> GAGCAGACCAG;> ACTCCACTCA;> CTAGT;> TCTGAGTGGGGTCTG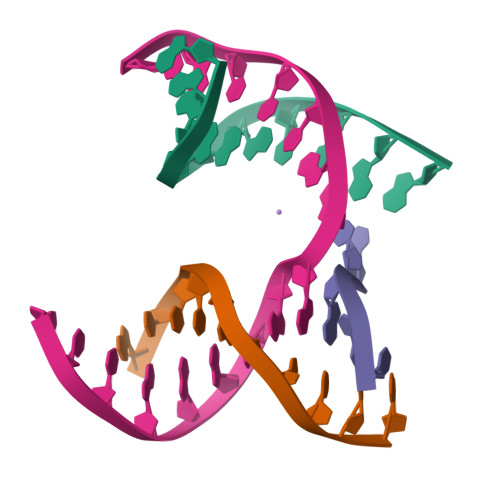C1-(4-{5-[(2E)-but-2-en-2-yl]thiophen-2-yl}phenyl)azetidine | C17 H19 N S | 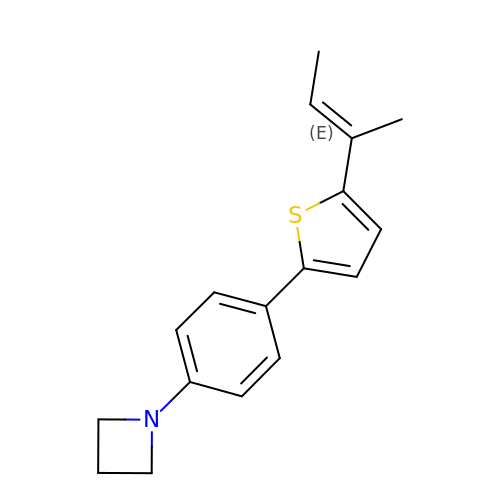UJDWZSVKXHLFTM-QLKAYGNNSA-N>[5x]MALVDGFLELERSSGKLEWSAILQKMASDLGFSKILFGLLPKDSQDYENAFIVGNYPAA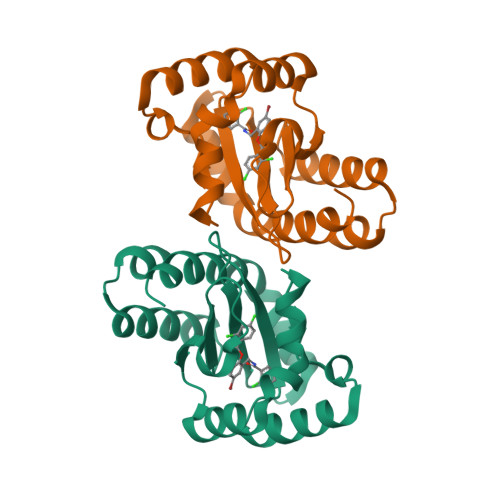WREHYDRAGYARVDPTVSHCTQSVLPIFWEPSIYQTRKQHEFFEEASAAGLVYGLTMPLHGARGELGALSLSVEAENRAEANRFMESVLPTLWMLKDYALQSGAGLAFEHPVSK> MLD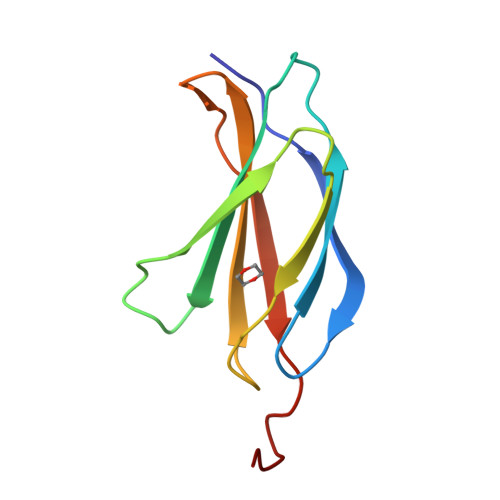APTDLQVTNVTDTSITVSWTPPSATITGYRITYTPSNGPGEPKELTVPPSSTSVTITGLTPGVEYVVSVYALKDNQESPPLVGTQTTGGHHHHHH>[4x]MKAIIVKPPNAGVQVKDVDEKKLDSYGKIKIRTIYNGICGADREIVNGKLTLSTLPKGKDFLVLGHEAIGVVEESYHGFSQGDLVMPVNRRGCGICRNCLVGRPDFCETGEFGEAGIHKMDGFMREWWYDDPKYLVKIPKSIEDIGILAQPLADIEKSIEEILEVQKRVPVWTCDDGTLNCRKVLVVGTGPIGVLFTLL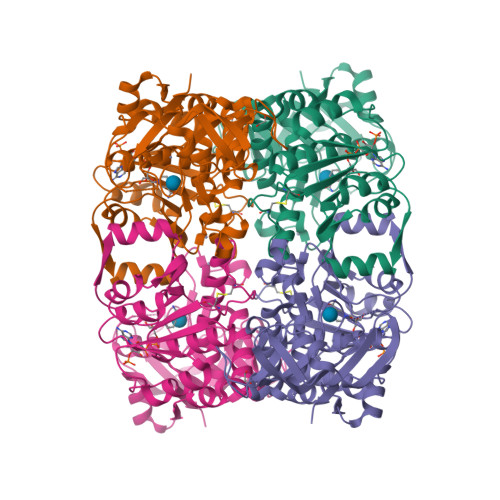FRTYGLEVWMANRREPTEVEQTVIEETKTNYYNSSNGYDKLKDSVGKFDVIIDATGADVNILGNVIPLLGRNGVLGLFGFSTSGSVPLDYKTLQEIVHTNKTIIGLVNGQKPHFQQAVVHLASWKTLYPKAAKMLITKTVSINDEKELLKVLREKEHGEIKIRILWE> MEDIEKIKPYVRSFSKALDELKPEIEKLTSKSLDEQLLLLSDERAKLELINRYAYVLSSLMFANMKVLGVKDMSPILGELKRVKSYMDKAKQYDNRITKSNEKSQAEQ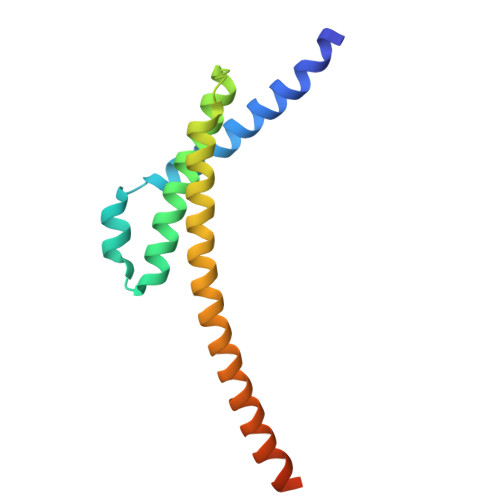EKAKNIISNVLDGNKNQFEPSISRS> GSHMQRVPLSVQLKPEVSPTQDIRLWVSVEDAQMHTVTIWLTVRPD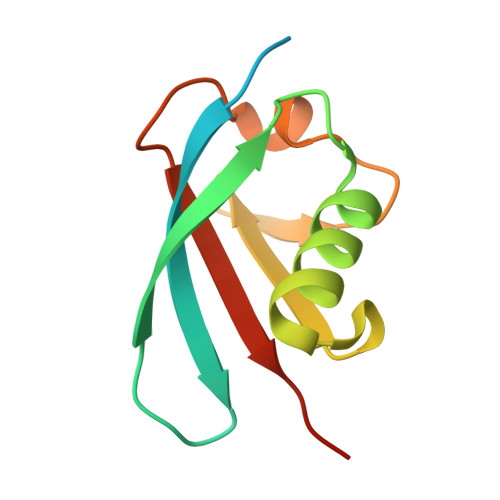MTVASLKDMVFLDYGFPPVLQQWVIGQRLARDQETLHSHGVRQNGDSAYLYLLSARNTS> MLRDLFDRAVVLSAYIHNLSSEMFSEFDKRYTHGRGFITKAINSCHTSSLATPEDKE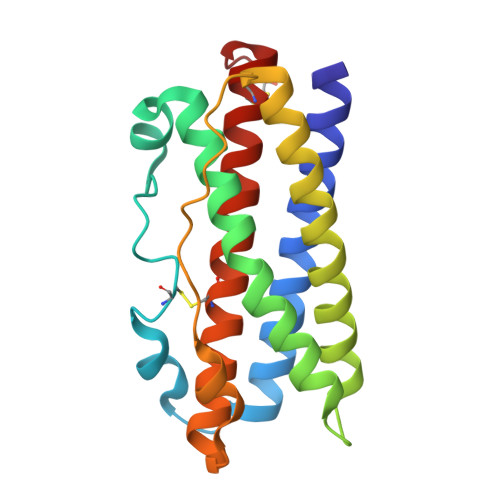QAQQMNQKDFLSLIVSILRSWNEPLYHLVTEVRGMQEAPEAILSKAVEIEEQTKRLLERMELIVSQVHPETKENEIYPVWSGLPSLQMADEESRLSAYYNLLHCLRRDSHKIDNYLKLLKCRIIHNNNC>[2x]HHHHHHMPLLTIGDQFPAYQLTALIGGDLSKVDAKQPGDYFTTITSDEHPGKWRVVFFWPKDFTFVCPTEIADF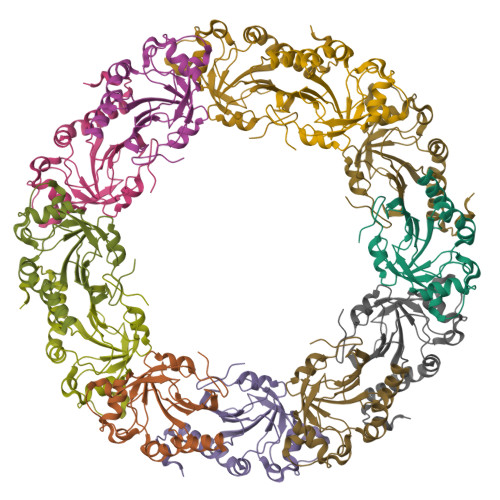SKLNDEFEDRDAQILGVSIDSEFAHFQWRAQHNDLKTLPFPMLSDIKRELSQAAGVLNADGVADRVTFIVDPNNEIQFVSATAGSVGRNVDEVLRVLDALQSDELCASNWRKGDPTLDAGELLKASA> MTVFRQENVDDYYDTGEELGSGQFAVVKKCREKSTGLQYAAKFIKKRRTKSSRRGVSREDIEREVSILKEIQHPNVITLHEVYENKTDVILILELVAGGELFDFLAEKESLTEEEATEFLKQILNGVYYLHSLQIAHFDLKPENIMLLDRNVPKPRIKI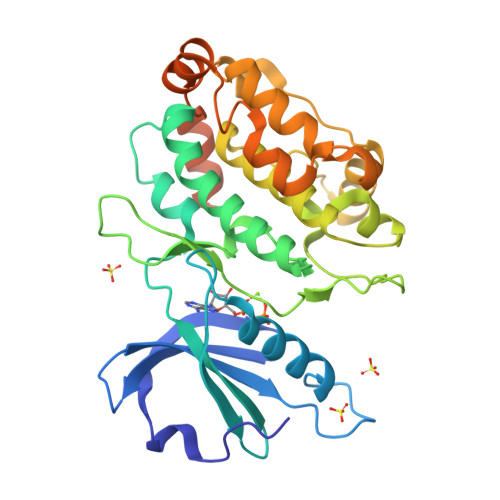IDFGLAHKIDFGNEFKNIFGTPAFVAPEIVNYEPLGLEADMWSIGVITYILLSGASPFLGDTKQETLANVSAVNYEFEDEYFSNTSALAKDFIRRLLVKDPKKRMTIQDSLQHPWIKPKDTQQALSRKASAVNMEKFKKFAARKKWKQSVRLISLCQRLSRSFLSRSNMSVARSD> MHHHHHHGMASMTARPLSELVERGWAAALEPVADQVAHMGQFLRAEIAAGRRYLPAGSNVLRA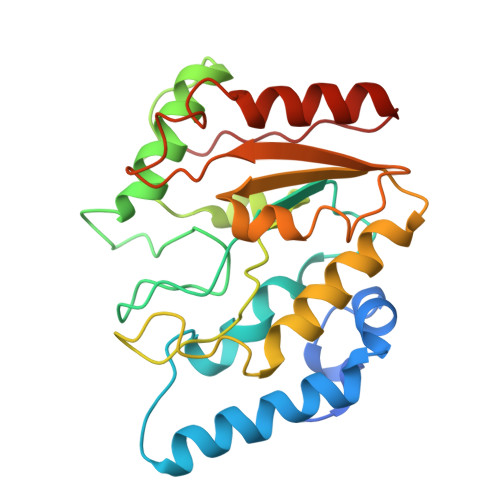FTFPFDNVRVLIVGQDPYPTPGHAVGLSFSVAPDVRPWPRSLANIFDEYTADLGYPLPSNGDLTPWAQRGVLLLNRVLTVRPSNPASHRGKGWEAVTECAIRALAARAAPLVAILWGRDASTLKPMLAAGNCVAIESPHPSPLSASRGFFGSRPFSRANELLVGMGAEPIDWRLP>MAPCLENVACVNLSAMPPAPPSPQPVSHKQAATLCRQGRTCALKSGSNESGGSVTSTYTSYRLISQDIGKSLERVSKQPDVARETEYYREKIGSVKSIDDFMADTRLYNYALKAHGLEDMAYAKAFIRKVLTEGASDKNAFANKLSDNRYAELAKSLDFAGLGAAATATEAAKSGVIGNYARQTLEQEAGDDNNGVRLALYFERKAPTIKSGLDFLADDALAQVFRTTFNLPDAFAAADVDKQAALIEKSINIKDLQDPEKVGKLLERFTIM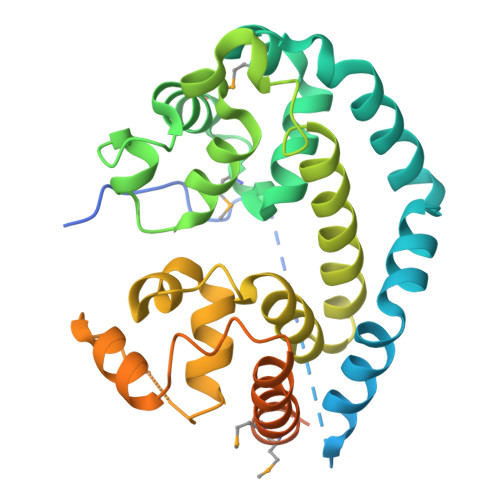WEMQNPSTTYDPLAVFGSSSGYGISPDLLISINSLKLGGKAAALEHHHHHH[2x]>GAMAVYPCGICTNEVNDDQDAILCEASCQKWFHRICTGMTETAYGLLTAEASAVWGCDTCMAD[2x];>GAMVYVFSTEMANKAAEAVLKGQVETIVSFHI[2x];>[2x]ARTKQTA

Pygo and BCL9/Legless transduce the Wnt signal by promoting the transcriptional activity of β-catenin/Armadillo in normal and malignant cells. Molecularly, BCL9/Lgs proteins function as adaptors between Pygo and Armadillo/β-catenin, by binding through their homology domain 1 (HD1) to the PHD finger in the C terminus of Pygo, and through their homology domain 2 (HD2) to the Armadillo repeat domain of Armadillo/β-catenin (Kramps et al., 2002; Städeli and Basler, 2005). We show that human and Drosophila Pygo PHD fingers associate with their cognate HD1 domains from BCL9/Legless to bind specifically to the histone H3 tail methylated at lysine 4 (H3K4me). Therefore, this is a prime example of histone tail binding by a PHD finger (of Pygo) being modulated by a cofactor (BCL9/Legless).

We truncated the N terminus of hPHD by seven residues to avoid this autoinhibition artifact, and crystallized this hPHD-HD1 complex with a 5× molar excess of a 9-mer H3K4me2 peptide (Kd, 11 μM), which allowed us to solve the structure of this ternary complex (Tern1) at 1.7 Å resolution. In both maps, we observed additional electron densities in the predicted histone-binding pockets of hPHD, which allowed us to model the first seven amino acids of the histone H3 tail bound to the hPHD-HD1 complex. The first five amino acids (A1–Q5) exhibit an extended conformation, with R2-K4me2 forming an antiparallel β sheet with PHD β3 (A356–L358), as observed in all other known PHD-H3K4me structures, while T6 and A7 meander off the PHD surface, looping back on itself, stabilized by an H bond between T6 and T3 (see also Ramon-Maiques et al., 2007). K4me2 and A1 occupy two adjacent cavities, separated by PHD W366. The K4me2 cavity consists of a semiaromatic cage with W366, Y341, and D352 forming the walls, and V350 and A356 the base. The two K4me2 methyl groups make hydrophobic interactions with W366 (in PHD β4) and Y341, while D352 (in the EVND motif) forms an H bond with the Nζ of the K4me2 side chain. This H bond could not be formed with K4me3 because the extra methyl group would preclude the approach of the D352 carboxyl group. Specifically, the N-terminal amino group of A1 is tightly bound to backbone carbonyl groups of L382, E385, and A388, as in all other PHD fingers. In the ternary complexes, the PHD groups around the K4me2 pocket close up slightly around the peptide (arrow 1) and the Pygo loop becomes more ordered.> GGLEKDFLPLAFGWFLTKKSSETLRKAGQVFLEELGNHKAFKKELRHFISGDEPKEKLELVSYFGKRPPGVLHCTTKFCDYGKAAGAEEYAQQEVVKRSYGKAFKLSISALFVTPKTAGAQVVLTDQELQLWPSDLDKPSASEGLPPGSRAHVTLGCAADVQPVQTGLDLLDILQQVKGGSQGEAVGELPRGKLYSLGKGRWMLSLTKKMEVKAIFTGYYG

2′,3′-cyclic nucleotide 3′-phosphodiesterase (CNPase) comprises 4% of total myelin protein in the central nervous system (CNS), being the most abundant CNS non-compact myelin protein4. CNPase consists of an N-terminal polynucleotide kinase-like domain10, a catalytic phosphodiesterase domain11, and a membrane-anchored C-terminal tail, which contains a cysteine residue that undergoes isoprenylation. The catalytic domain enables the rapid hydrolysis of nucleoside 2′,3′-cyclic phosphates to nucleoside 2′-phosphates. The CNPase catalytic site, lying in a groove between two lobes, has pseudo two-fold symmetry and contains two apposing His-X-Thr-X (X denotes a hydrophobic residue) motifs, characteristic for 2H phosphoesterases 113537.

Tyr168 is one of the aromatic residues on the CNPcat surface that we suggested to form a binding surface for RNA34. Tyr168 interacts with the substrate ribose moiety through C-H…π hydrogen bonding. We carried out mutagenesis to study the role of the aromatic side chain of Tyr168. While the Y168A mutation decreases catalytic activity, Y168S retains it, albeit with an elevated KM compared to the wild-type enzyme. In the absence of the aromatic ring, the serine OH group appears to be enough to retain catalytic activity; this could be related to differences in water networks or overall dynamics in Y168A and Y168S. In the mutants, the missing ion-dipole interaction between the Tyr168 hydroxyl group and the His230 imidazole ring apparently causes His230 and Ala/Ser168 to reposition in the active site by ~1 Å. Additionally, loop α3-β2 moves towards the active site by the same distance. These structural features suggest that Tyr168 also has a role in fine-tuning the active site conformation with its bulkiness.> EPQHNVMQMGGDFANNPNAQQFIDKMVNKHGFDRQQLQEILSQAKRLDSVLRLMDNQAPTTSVKPPSGPNGAWLRYRKKFITPDNVQNGVVFWNQYEDALNRAWQVYGVPPEIIVGIIGVETRWGRVMGKTRILDALATLSFNYPRRAEYFSGELETFLLMARDEQDDPLNLKGSFAGAMGYGQFMPSSYKQYAVDFSGDGHINLWDPVDAIGSVANYFKAHGWVKGDQVAVMANGQAPGLPNGFKTKYSISQLAAAGLTPQQPLGN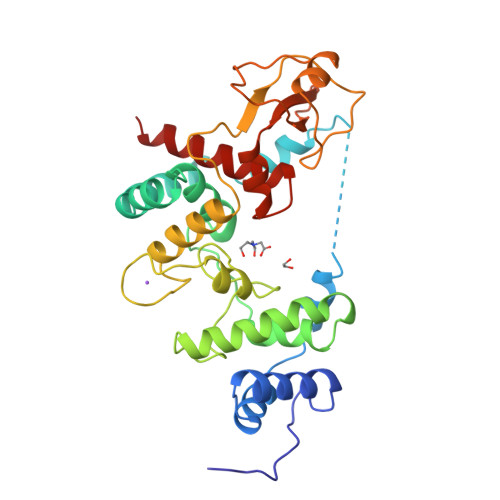HQQASLLRLDVGTGYQYWYGLPNFYTITRYNHSTHYAMAVWQLGQAVALARVQ> GSSGS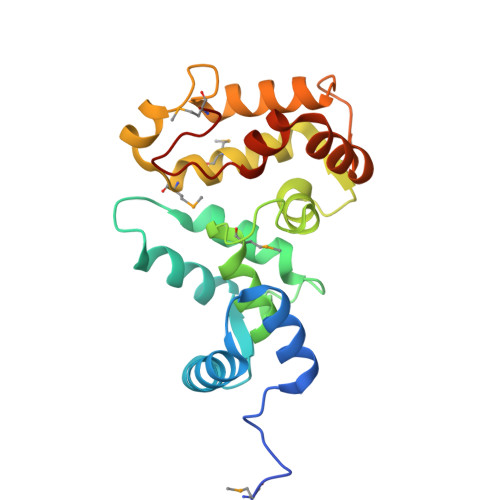SGMGNSKSGALSKEILEELQLNTKFSEEELCSWYQSFLKDCPTGRITQQQFQSIYAKFFPDTDPKAYAQHVFRSFDSNLDGTLDFKEYVIALHMTTAGKTNQKLEWAFSLYDVDGNGTISKNEVLEIVMAIFKMITPEDVKLLPDDENTPEKRAEKIWKYFGKNDDDKLTEKEFIEGTLANKEILRLIQFEPQKVKEKMKNA>[2x]TSIPGGWTRQDPTEARFLELAHFATSSQTE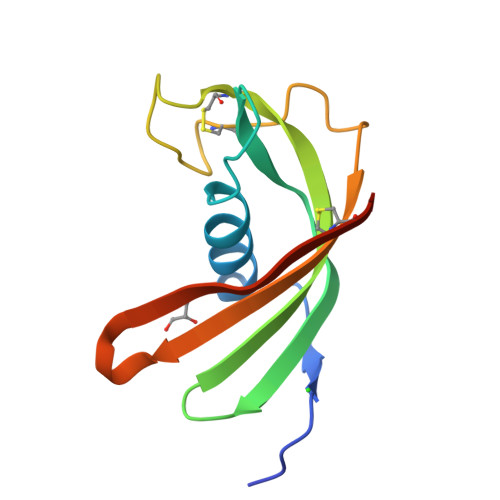GREFYDTVVTVKEVETQVVAGMNYKLTIEISPSVCKIGEVQYSAEQCVPKDAQQKSTCVAVIYHVPWQNQKSVTSYRCEHHHHHH> PLEEAFDWDEYPVQRVTATGYTA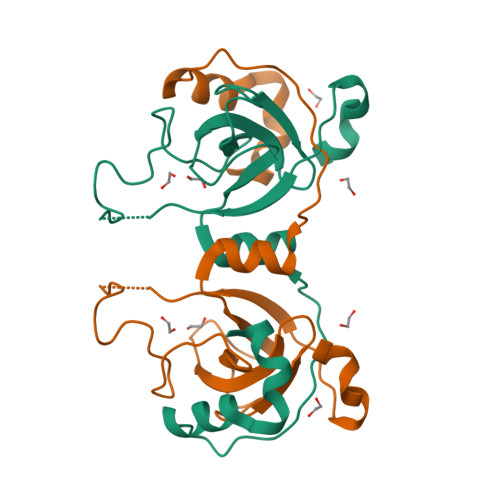GAESTGKNPGDPLYGLTYSGVKVKRDLYSTVAADPSVFPIGTILFIPNYGLGVVADTGSAIKGNRLDLYFETVKDVYNEWGKKTLDVYVIKKGTGKITEDELEKLNETKSLQVFRNQYKTVKE>GAMETLHITKTMKNIEVPETKTASFECEVSHFNVPSMWLKNGVEIEMSEKFKIVVQ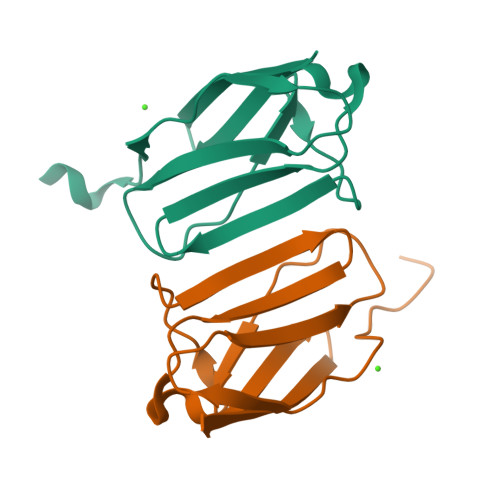GKLHQLIIMNTSTEDSAEYTFVCGNDQVSATLTVT[16x]> GSHMTPKDDEFYQQWQLKYPKLILREASSVSEELHKEVQEAFLTLHKHGCLFRDLVRIQGKDLLTPVSRILIGNPGCTYKYLNTRLFTVPWPVKGSNIKHTEAEIAAACETFLKLNDYLQIETIQALEELAAKEKANEDAVPLCMSADFPRVGMGSSYNGQDEVDIKSRAAYNVTLLNFMDPQKMPYLKEEPYFGMGKMAVSWHHDENLVDRSAVAVYSYSCEGPEEESEDDSHLEGRDPD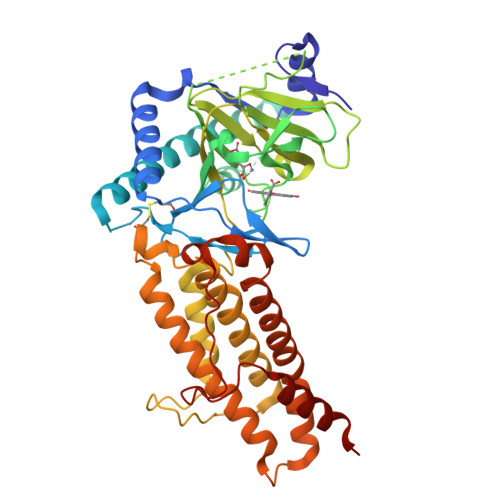IWHVGFKISWDIETPGLAIPLHQGDCYFMLDDLNATHQHCVLAGSQPRFSSTHRVAECSTGTLDYILQRCQLALQNVCDDVDNDDVSLKSFEPAVLKQGEEIHNEVEFEWLRQFWFQGNRYRKCTDWWCQPMAQLEALWKKMEGVTNAVLHEVKREGLPVEQRNEILTAILASLTARQNLRREWHARCQSRIARTLPADQKPECRPYWEKDDASMPLPFDLTDIVSELRGQLLEAKP> MASDMEEKFREAFILFSSCSDHIEMYKFFELMNSFGIILTND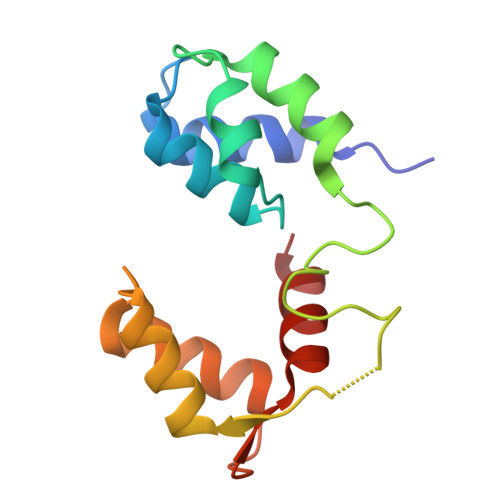EKAALPNDINMDYWLNFAKKHYNYEQPFKHINNVNEQNTNVQIKIDNFLGIMKALDTRLTESDLNILLQITNPENKSTLNLKTVSQKLTESI> MKKEPIKMPNPDNTEAYVAGEVAIENSAIALSGIVSVANNADNRLEVFGVSTDSAVWHNWQTAPLPNSSWAGWNKFNGVVTSKPAVHRNSDGRLEVFVRSTDNALWHNWQTAADTNTWSSWQPLYGGITSNPEVCLNSDGRLEVFARGTDNALWHIWQTAAHTNSWSNWKSLGGTLTSNPAAHINADGRIEVFARGADNALWHIWQTAAHTDQWSNWQSLKSVITSDPVVIGNCDGRLEVFARGADNTLRHISQIGSDSVSWSNWQCLDGVITSAPAAVKNISGRLEVFARGADNTLWRTWQTSQNGPWSNWSSFTGIIASAPTVAKNSDGRIEVFVLGLDKALWHLWQTTSSTTSSWTTWALIGGITLIDASVIK

In this article, we studied five members of the PLL lectin family from P. laumondii subsp. laumondii TT01 (PLL, PLL2, PLL3, PLL4, PLL5, collectively referred to as PLLs). All studied lectins belong to the seven-bladed β-propeller structural family. Each blade makes a W-motif composed of four antiparallel beta-strands (β1-β4) connected by β-turns and loops. The saccharide binding sites are located between the adjacent blades and are uniquely organized in two separate circles around the monomer.

In this study, we used PLL originating directly from P. laumondii subsp. laumondii TT01 (formerly P. luminescens subsp. laumondii TT01) to ensure all five studied lectins originate from the same bacterial strain. The two versions of PLL differ in 12 mutated amino acids – five of them affecting three potential binding sites. Additionally, the protein used in this study lacks the His-tag on the C-terminus and is seven residues longer on the N-terminus. PLL is a homotetramer stabilized by up to four disulphide bridges. The electron density for the Cys267-Cys267 bridge shows one possible orientation of cysteines with sulphur atoms in 2.35 Å distance, corresponding to disulphide bond formation. Cys234 can adopt two different conformations, which can be explained as a mixture of oxidised and reduced states. Therefore Cys234-Cys234 bridge might not be formed in all PLL molecules. Our data from mass spectrometry (intact mass analysis) suggest the formation of both disulphide bridges, as PLL behaved as a covalent tetramer during this experiment. The PLL chain A blade W1 interacts with chain B blade W3, whereas in the case of PLL2, PLL4 and PLL5, chain A blade W1 interacts with chain B blade W5. For PLL and PLL4, only hydrophobic site activity has been shown, as αMeFuc occupied only H sites, and structure in complex with other potential ligands is not available.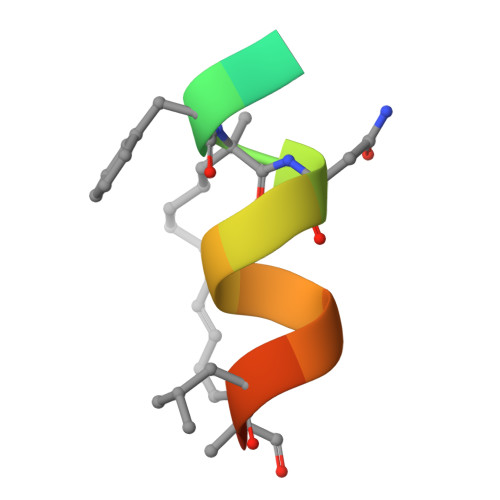> QSQQTFXNLWRLLLQN1-[2-chloranyl-7-[(1~{S})-1-methoxyethyl]pyrazolo[1,5-a]pyrimidin-6-yl]-3-(5-chloranyl-6-pyrrolidin-1-ylcarbonyl-pyridin-3-yl)urea | C20 H21 Cl2 N7 O3 | 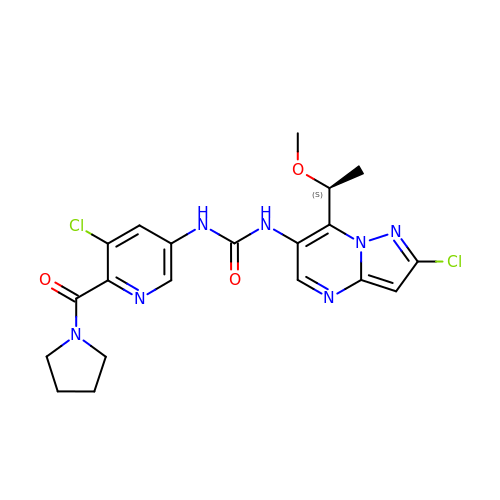OJTGJRAKRGEDPI-NSHDSACASA-N>MPKPINVRVTTMDAELEFAIQPNTTGKQLFDQVVKTVGLREVWFFGLQYVDSKGYSTWLKLNKKVTQQDVKKENPLQ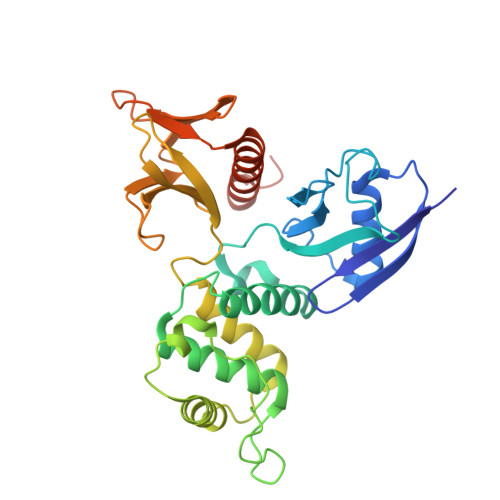FKFRAKFFPEDVSEELIQEITQRLFFLQVKEAILNDEIYCPPETAVLLASYAVQAKYGDYNKEIHKPGYLANDRLLPQRVLEQHKLTKEQWEERIQNWHEEHRGMLREDSMMEYLKIAQDLEMYGVNYFEIKNKKGTELWLGVDALGLNIYEHDDKLTPKIGFPWSEIRNISFNDKKFVIKPIDKKAPDFVFYAPRLRINKRILALCMGNHELYMRRRKPDTIEVQQMKAQAR[2x]>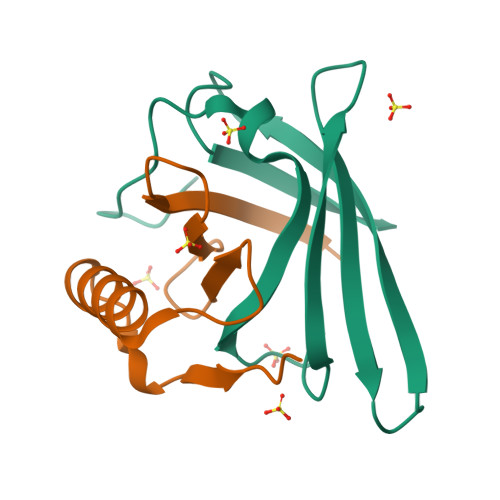[3x]MGHHHHHHLESTSLYKKSSSTPPRGVTVVNNFDAKRYLGTWYEIARFDHRFERGLEKVTATYSLRDDGGLNVINKGYNPDRGMWQQSEGKAYFTGAPTRAALKVSFF;>[3x]MGPFYGGYNVIALDREYRHALVCGPDRDYLWILSRTPTISDEVKQEMLAVATREGFDVSKFIWVQQPGS>MKTIIINGVQFNTDEDTTILKFARDNNIDISALCFLNNCNNDINKCEICTVEVEGTGLVTACDTLIEDGMIINTNSDAVNEKIKSRISQLLDIHEFKCGPCNRRENCEFLKLVIKYKARASKPFLPKDKTEYVDERSKSLTVDRTKCLLCGRCVNACGKNTETYAMKFLNKNGKTIIGAEDEKCFDDTNCLLCGQCIIACPVAALSEKSHMDRVKNALNAPEKHVIVAMAPSVRASIGELFNMGFGVDVTGKIYTALRQLGFDKIFDINFGADMTIMEEATELVQRIENNGPFPMFTSCCPGWVRQAENYYPELLNNLSSAKSPQQIFGTASKTYYPSISGLDPKNVFTVTVMPCTSKKFEADRPQMEKDGLRDIDAVITTRELAKMIKDAKIPFAKLEDSEADPAMGEYSGAGAIFGATGGVMEAALRSAKDFAENAELEDIEYKQVRGLNGIKEAEVEINNNKYNVAVINGASNLFKFMKSGMINEKQYHFIEVMACHGGCVNGGGQPHVNPKDLEKVDIKKVRASVLYNQDEHLSKRKSHENTALVKMYQNYFGKPGEGRAHEILHFKYKKSAWSHPQFK[2x]

[FeFe]-hydrogenases are nature's fastest catalysts for the evolution or oxidation of hydrogen. The complex Fe2[μ-(SCH2)2X](CN)2(CO)42– with X = NH was shown to integrate into the apo-form of [FeFe]-hydrogenases to yield a fully active enzyme. We herein report the structure of the [FeFe]-hydrogenase CpI from Clostridium pasteurianum in the unmaturated apo-form and the first high resolution structure of a fully active semisynthetic [FeFe]-hydrogenase along with the structures of three non-natural inactive derivatives of this [FeFe]-hydrogenase with changes in the inorganic active site. In contrast to already known structures of native CpI,3,30,39 the space group of the crystals was P21 for all five enzymes and the asymmetric units each contained two nearly identical molecules.

In this study we aim to expand the knowledge about maturation of [FeFe]-hydrogenases by reporting the crystal structure of the [FeFe]-hydrogenase from Clostridium pasteurianum (CpI) in its apo-form without the 2FeH-cluster (apoCpI). The crystal structure of apoCpI reported here is strikingly similar to structures of active CpI, both native and semisynthetic. The overall RMSD of the backbone atoms of apoCpI and native CpI30 is as low as 0.3 Å, while apoCpI and CpIADT display an RMSD of 0.4 Å over all backbone atoms (Table S1†). Significant differences in side-chain orientation are mainly limited to surface exposed residues with V423 being a notable exception. This residue in the central cavity is adapting a different rotamer, supposedly stabilized by one of the water molecules in the binding pocket for 2FeH. The structure of apoCpI presented here shows the three regions 405–423 (“plug”), 437–453 (“lid”) and 529–540 (“lock”) clearly in a “closed” conformation nearly identical to active CpI. Prominently, F417 in direct contact to the 2FeH-subcluster shows minimal deviation in apoCpI when compared to CpIADT, while it is moved by 15 Å in apoHydA1. Being devoid of the 2FeH-cluster, the active site binding pocket of apoCpI is occupied by seven water molecules and a chloride ion instead. Note that this leaves a water filled cavity of roughly 10 Å diameter in the center of the protein. Washed and subsequently dissolved crystals of apoCpI could be maturated with the synthetic ADT-bridged [2Fe] cluster to an activity of 1250 nmol H2/min/crystal, reassuring that the reported closed structure of apoCpI is not a dead-end conformation.> VPRGSAKGDGVTDDTAALTSALNDTPVGQKINGNGKTYKVTSLPDISRFINTRFVYERIPGQPLYYASEEFVQGELFKITDTPYYNAWPQDKAFVYENVIYAPYMGSDRHGVSRLHVSWVKSGDDGQTWSTPEWLTDLHPDYPTVNYHCMSMGVCRNRLFAMIETRTLAKNALTNCALWDRPMSRSLHLTGGITKAANQRYATIHVPDHGLFVGDFVNFSNSAVTGVSGDMTVATVIDKDNFTVLTPNQQTSDLNNAGKNWHMGTSFHKSPWRKTDLGLIPSVTEVHSFATIDNNGFAMGYHQGDVAPREVGLFYFPDAFNSPSNYVRRQIPSEYEPDASEPCIKYYDG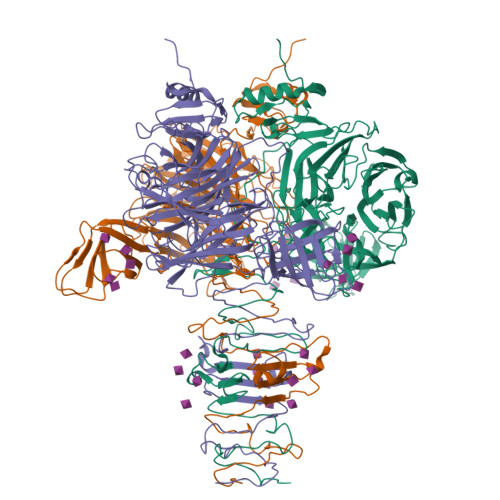VLYLITRGTRGDRLGSSLHRSRDIGQTWESLRFPHNVHHTTLPFAKVGDDLIMFGSEAAENEWEAGAPDDRYKASYPRTFYARLNVNNWNADDIEWVNITDQIYQGGIVNSGVGVGSVVVKDNYIYYMFGGEDHFNPWTYGDNSAKDPFKSDGHPSDLYCYKMKIGPDNRVSRDFRYGAVPNRAVPVFFDTNGVRTVPAPMEFTGDLGLGHVTIRASTSSNIRSEVLMEGEYGFIGKSIPTDNPAGQRIIFCGGEGTSSTTGAQITLYGANNTDSRRIVYNGDEHLFQSADVKPYNDNVTALGGPSNRFTTAYLGSNPIVT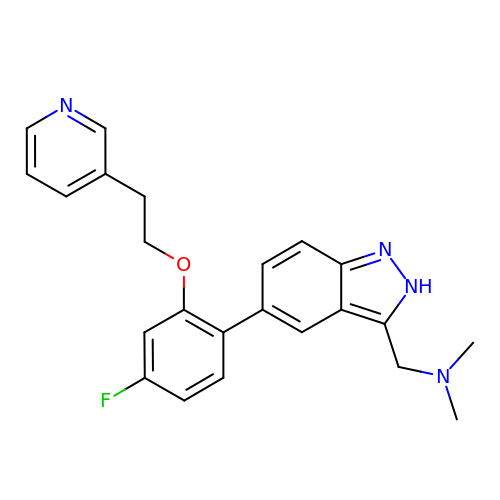[(5-{4-fluoro-2-[2-(pyridin-3-yl)ethoxy]phenyl}-1H-indazol-3-yl)methyl]dimethylamine | C23 H23 F N4 O | RNWBRNZKOWMEPZ-UHFFFAOYSA-N> MEKKDLIIRVAGEGGEGIISSGDFIAAACARAGLEVYTFKTFPAEIKGGYAMYQVRASSEKLYCQGDTFDVFCAFNGEAYEQNKDKIKPGTAFVYDYPGGDFEPDEIPEGVFAYPIPMSQTAKEMKSYRSKNMVALGALSELFNISENTLKEVLSDKFGKKGEEVLAFNLEAFDKGKALAKALTKADPFRVADPQEPKDVIIMAGNDAVGLGGILGGLEFFSAYPITPATEVAKYVATHLPKCGGDLVQAEDEIASIAQVLGASYAGKKSMTATSGPGLALMSEMLGMAHMSETPCLVVDVQRGGPSTGLPTKHEQSDLFLAIHGGHGDSPRIVLSVEDVKDCISMTVDGLNLAEKYQAPVIVLSDG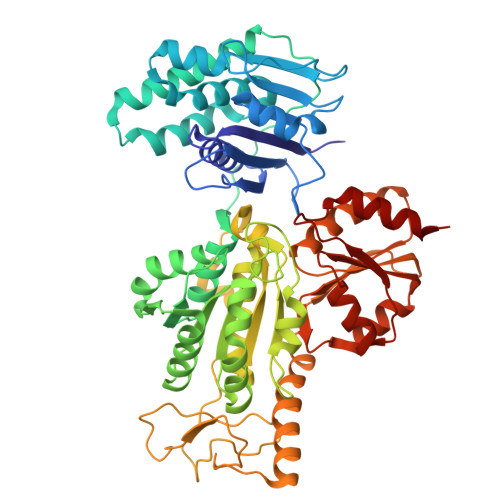SLAFSTQTIPRPKPEDFTIINRKTWDGQGTYKRYELTEDNISPMAAPGTPNAKHIATGLEHGETGAPNYSPANHELMHRKRFNKQNSVLDFYKNMEVEGVEGEADVGIITWGSTIGVVREAMQRLTAEGLKVKAMYPKLLWPMPVADYDAFGATCKKVIVPEVNFQGQLSHFIRAETSIKPIPYTICGGLPFTPEMIVNRVKEEIQ>CGIVGAIAQRDVAEILLEGLRRLEYRGYDSAGLAVVDAEGHMTRLRRLGKVQMLAQAAEEHPLHGGTGIAHTRWATHGEPSEVNAHPHVSEHIVVVHNGIIENHEPLREELKARGYTFVSETDTEVIAHLVNWELKQGGTLREAVLRAIPQLRGAYGTVIMDSRHPDTLLAARSGSPLVIGLGMGENFIASDQLALLPVTRRFIFLEEGDIAEITRRSVNIFDKTGAEVKRQ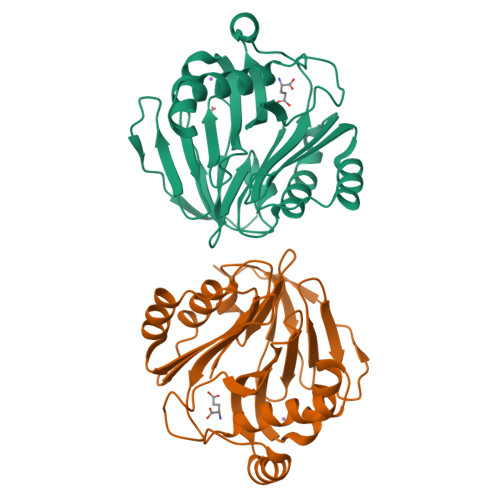DIESNLQY[2x]> GRLVGLELSNFKSYRGVTKVGFGESNFTSIIGPNGSGKSNMMDAISFVLGVRSNHLRSNILKDLIYRGVLSNPQSAYVKAFYQKGNKLVELMRIISRNGDTSYKIDGKTVSYKDYSIFLENENILIKAKNFLVFQGDVEQIAAQSPVELSRMFEEVSGSIQYKKEYEELKEKIEKLSKSAEEKKILNQFLKIKKKRKELFEKTFDYVSDHLDAIYRELTKNPNSNVELAGGNASLTIEDEDEPFNAGIKYHATPPLKRFKDMEYLSGGEKTVAALALLFAINSYQPSPFFVLDQVDAALDITNVQRIAAYIRRHRNPDLQFIVISLKNTMFEKSDALVGVYRQQQENSSKIITLDLSNYA;> GPYIKRVIIKGFKTYRNETIIDNFSPHQNVIIGSNGSGKSNFFAAIRFVLSDDYSNLKREERQGLIHQGSGGSVMSASVEIVFHDPDHSMILPSGVLSRGDDEVTIRRTVGLKKDDYQLNDRNVTKGDIVRMLETAGFSMNNPYNIVPQGKIVALTNAKDKERLQLLEDVVGAKSFEVKLKASLKKMEETEQKKIQINKEMGELNSKLSEMEQERKELEKYNELERNRKRAFENFKKFNERRKDLAERASELDESKDSIQDLIVKLKQQKVNAVDSTFQKVSENFEAVFERLVPRGTAKLIIHRYTGVSISVSFNSKQNEQLHVEQLSGGQKTVCAIALILAIQMVDPASFYLFDQIDAALDKQYRTAVATLLKELSKNAQFICTTFRTDMLQVADKFFRVKYENKISTVIEVNREEAIGFIR;> TLRTSGELLQGIVRVYSKQATFLLTDIKDTLTKISMLVIFTDVLKSITKREASRGFFDILSLATEGCIGLSQTEAFGNIKIDA;> MSYPGKDKNIPGRIIEALEDLPLSYLVPKDGLAALVNAPMRVSLPFDKTIFTSADDGRDVNINVLGTANSTTSSIKNEAEKERLVFKRPSNFTSSANSVDYVPTNFLEGLSPLAQSVLSTHKGLNDSINIEKKSEIVSRPEAKHKLESVTSNAGNLSFNDNSSNKKTKTSTGVTMTQANLAEQYLNDLKNILDIVGFDQNSAEIGNIEYWLQLPNKKFVLTTNCLTKLQMTIKNITDNPQLSNSIEITWLLRLLDVMVCNIKFSKSSLKMGLDDSMLRYIALLSTIVLFNIFLLGKNDSNLHRESYIMEPVNFLSDLIESLKILTIEYGSLKIEFDTFQEALELLPKYIRNGPFLDDNVTAKLVYIFSDLLMNNDIEATTNIQFQSFWDNVKRISSDILVSLFGSFDQQRGFIIEELLSHIEKLPTKRIQKKLRKVGNQNIYITDFTFTLMSMLENINCYSFCNQMKDIAPENIDLLKNEYKKQEEFLFNIVEHINDTILERFFKNPSALRYVIDNFVQDLLLLISSPQWPVTEKILSSLLKRLLSVYSPSMQVSANIETICLQLIGNIGSTIFDIKCSTRDHEDNNLIKMINYPETLPHFFKSFEECIAYNETIKCRRSATRFLWNLRLGTILILEEYTKDAKEQIITVDNELKKILEQIKDGGLGPELENREADFSTIKLDYFSILHAFELLNLYDPYLKLILSLLAKDKIKLRSTAIKCLSMLASKDKVILSNPMVKETIHRRLNDSSASVKDAILDLVSINSSYFEFYQQINNNYNDDSIMVRKHVLRINEKMYDETNDIVTKVYVIARILMKIEDEEDNIIDMARLI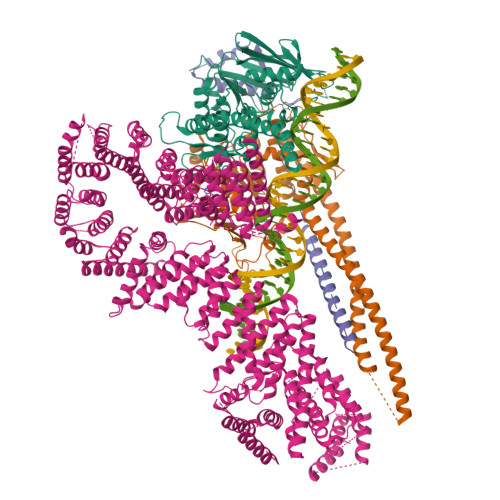LLNRWILKVHEVLDQPEKLKEISSSVLLVMSRVAIMNEKCSQLFDLFLNFYLLNKEAHSKEAYDKITHVLTILTDFLVQKIVELNSDDTNEKNSIVDKQNFLNLLAKFADSTVSFLTKDHITALYPYMVSDEKSDFHYYILQVFRCTFEKLANFKQKFLYDLETTLLSRLPKMNVREIDEAMPLIWSVATHRHDTARVAKACSSCLSHLHPYINKANNEEAAIVVDGKLQRLIYLSTGFARFCFPKPSNDKIAFLQEGETLYEHITKCLLVLSKDKITHVIRRVAVKNLTKLCGNHPKLFNSRHVLHLLDKEFQSDQLDIKLVILESLYDLFLLEERKSVRNTGVNSTLSSNSILKKKLLKTNRVEFANDGVCSALATRFLDNILQLCLLRDLKNSLVAIRLLKLILKFGYTNPSHSIPTVIALFASTSQYIRHVAYELLEDLFEKYETLVFSSLSRGVTKAIHYSIHTDEKYYYKHDHFLSLLEKLCGTGKKNGPKFFKVLKRIMQSYLDDITDLTSTNSSVQKSIFVLCTNISNITFVSQYDLVSLLKTIDLTTDRLKEVIMDEIGDNVSSLSVSEEKLSGIILIQLSLQDLGTYLLHLYGLRDDVLLLDIVEESELKNKQLPAKKPDISKFSAQLENIEQYSSNGKLLTYFRKHVKDT>GSMSSERVLSYAPAFKSFLDTSFFQELSRLKLDVLKLDSTCQPLTVNLDLHNIPKSADQVPLFLTNRSFEKHNNKRTNEVPLQGSIFNFNVLDEFKNLDKQLFLHQRALECWEDGIKDINKCVSFVIISFADLKKYRFYYWLGVPCFQRPSSTVLHVRPEPSLKGLFSKCQKWFDVNYSKWVCILDADDEIVNYDKCIIRKTKVLAIRDTSTMENVPSALTKNFLSVLQYDVPDLIDFKLLIIRQNEGSFALNATFASIDPQSSSSNPDMKVSGWERNVQGKLAPRVV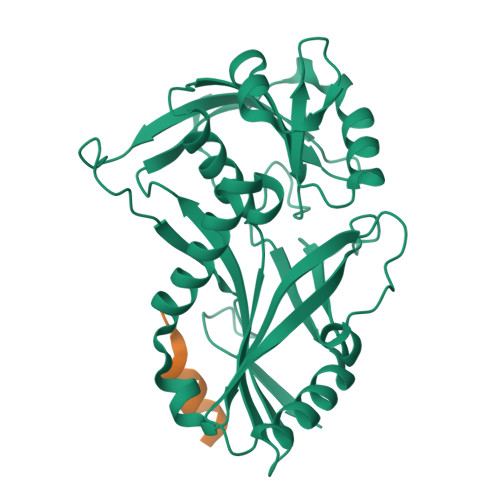DLS[2x];>SIDDIDELIQDMEIKEE[2x]naphthalen-2-ylmethanol 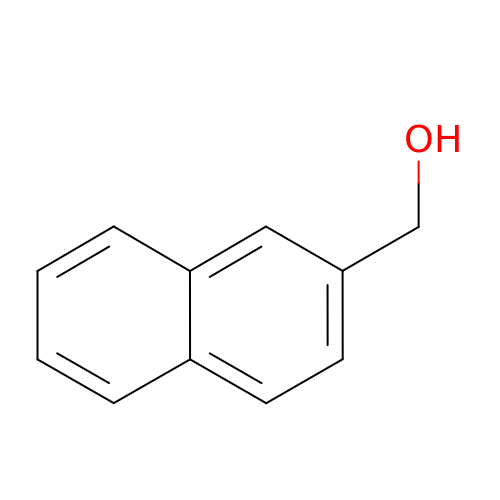| C11 H10 O | MFGWMAAZYZSWMY-UHFFFAOYSA-N7-(2-ethoxynaphthalen-1-yl)-6-methylquinazoline-2,4-diamine | C21 H20 N4 O | 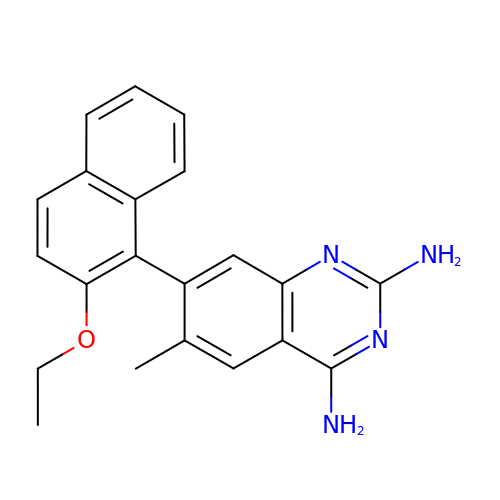DYQBRXOQGFCHCN-UHFFFAOYSA-N> GSYCPRN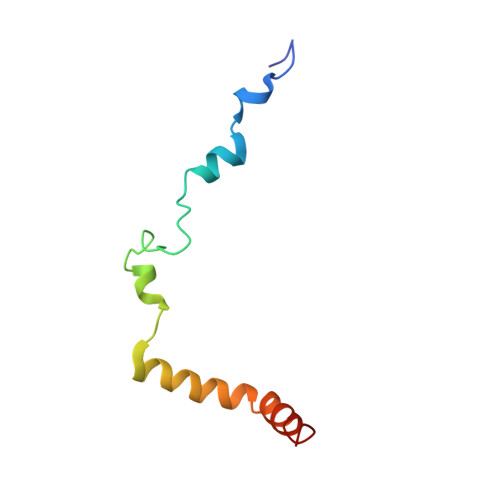LHLLPTTDTYLSKVSDDPDNLEDVDDEELNAHLLNEEASKLKERIWIGLNADFLLEQESKRLKQE>[4x]MRKLNPALEFRDFIQVLKDEDDLIEITEEIDPNLEVGAIMRKAYESHLPAPLFKNLKGASKDLFSILGCPAGLRSKEKGDHGRIAHHLGLDPKTTIKEIIDYLLECKEKEPLPPITVPVSSAPCKTHILSEEKIHLQSLPTPYLHVSDGGKYLQTYGMWILQTPDKKWTNWSIARGMVVDDKHITGLVIKPQHIRQIADSWAAIGKANEIPFALCFGVPPA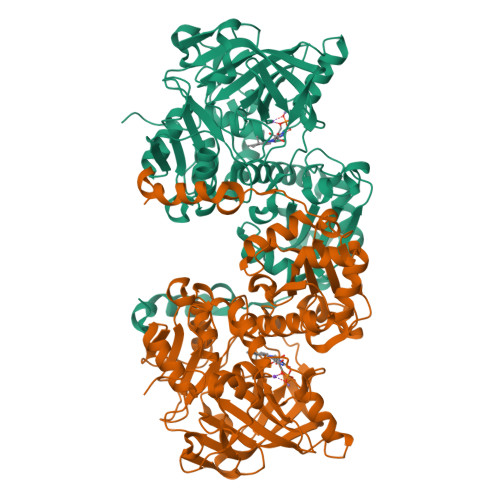AILVSSMPIPEGVSESDYVGAILGESVPVVKCETNDLMVPATSEMVFEGTLSLTDTHLEGPFGDMHGYVFKSQGHPCPLYTVKAMSYRDNAILPVSNPGLCTDETHTLIGSLVATEAKELAIESGLPILDAFMPYEAQALWLILKVDLKGLQALKTTPEEFCKKVGDIYFRTKVGFIVHEIILVADDIDIFNFKEVIWAYVTRHTPVADQMAFDDVTSFPLAPFVSQSSRSKTMKGGKCVTNCIFRQQYERSFDYITCNFEKGYPKGLVDKVNENWKRYGYKHHHHHH> MARRNRRLSSASVYRYYLKRISMNIGTTGHVNGL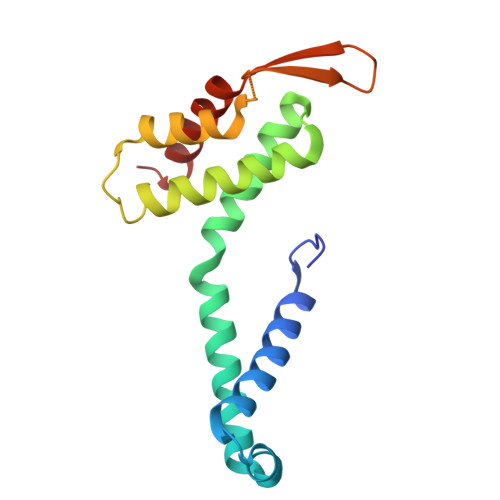SIAGNPEIMRAIARLSEQETYNWVTDYAPSHLAKEVVKQISGKYNIPGAYQGLLMAFAEKVLANYILDYKGEPLVEIHHNFLWELMQRQSGAGLGVTSGFIYTFVRKDGKPVTVDMSKVLTEIEDALFKLVKK> GPGSMTTRSARVIIASTRASSGEYEDRCGPIITEWLAQQGFSSAQPEVVA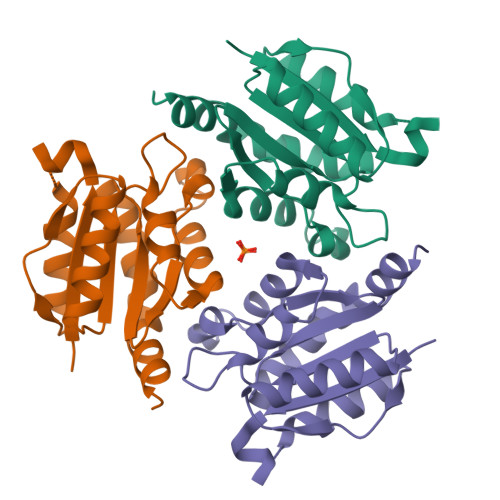DGSPVGEALRKAIDDDVDVILTSGGTGIAPTDSTPDQTVAVVDYLIPGLAEAIRRSGLPKVPTSVLSRGVCGVAGQTLIVNLPGSPGGVRDGLGVLAGVLDHALDQLAGKDHPR>[2x]GSGLPFLVQRTVARQITLLECVGKGRYGEVWRGSWQGENVAVKIFSSRDEKSWFRETELYNTVMLRHENILGFIASDMTSRHSSTQLWLITHYHEMGSLYDYLQLTTLDTVSCLRIVLSIASGLAHLHIEIFGTQGKPAIAHRDLKSKNILVKKNGQCCIADLGL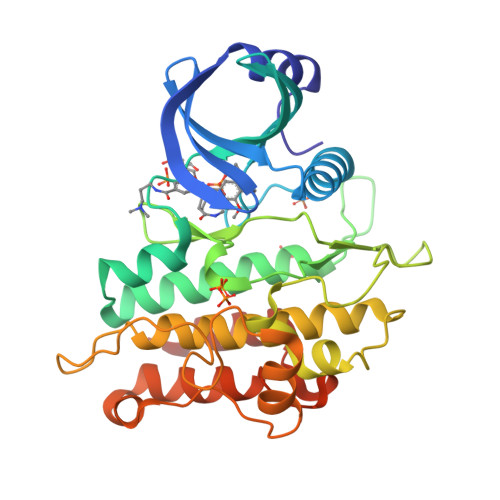AVMHSQSTNQLDVGNNPRVGTKRYMAPEVLDETIQVDCFDSYKRVDIWAFGLVLWEVARRMVSNGIVEDYKPPFYDVVPNDPSFEDMRKVVCVDQQRPNIPNRWFSDPTLTSLAKLMKECWYQNPSARLTALRIKKTLTKIDNSLDKLKTDC> MSDNRRRRREEDDSDSENELPPSSPQQHFRGGMNPVSSPIGSPDMINPEGDDNEVDDVPDIDEVEEQMNEVDLMDDNMYEDYAADHNRDRYDPDQVDDREQQELSLSERRRIDAQLNERDRLLRNVAYIDDEDEEQEGAAQLDEMGLPVQRRRRRRQYEDLENSDDDLLSDMDIDPLREELTLESLSNVKANSYSEWITQPNVSRTIARELKSFLLEYTDETGRSVYGARIRTLGEMNSESLEVNYRHLAESKAILALFLAKCPEEMLKIFDLVAMEATELHYPDYARIHSEIHVRISDFPTIYSLRELRESNLSSLVRVTGVVTRRTGVFPQLKYVKFNCLKCGSILGPFFQDSNEEIRISFCTNCKSKGPFRVNGEKTVYRNYQRVTLQEAPGTVPPGRLPRHREVILLADLVDVSKPGEEVEVTGIYKNNYDGNLNAKNGFPVFATIIEANSIKRREGNTANEGEEGLDVFSWTEEEEREFRKISRDRGIIDKIISSMAPSIYGHRDIKTAVACSLFGGVPKNVNGKHSIRGDINVLLLGDPGTAKSQILKYVEKTAHRAVFATGQGASAVGLTASVRKDPITKEWTLEGGALVLADKGVCLIDEFDKMNDQDRTSIHEAMEQQSISISKAGIVTTLQARCSIIAAANPNGGRYNSTLPLAQNVSLTEPILSRFDILCVVRDLVDEEADERLATFVVDSHVRSHPENDEDREGEELKNNGESAIEQGEDEINEQLNARQRRLQRQRKKEEEISPIPQELLMKYIHYARTKIYPKLHQMDMDKVSRVYADLRRESISTGSFPITVRHLESILRIAESFAKMRLSEFVSSYDLDRAIKVVVDSFVDAQKVSVRRQLRRSFAIYTLGH;> MEGSTGFDGDATTFFAPDAVFGDRVRRFQEFLDTFTSYRDSVRSIQVYNSNNAANYNDDQDDADERDLLGDDDGDDLEKEKKAASSTSLNILPHRIIISLDDLREFDRSFWSGILVEPAYFIPPAEKALTDLADSMDDVPHPNASAVSSRHPWKLSFKGSFGAHALSPRTLTAQHLNKLVSVEGIVTKTSLVRPKLIRSVHYAAKTGRFHYRDYTDATTTLTTRIPTPAIYPTEDTEGNKLTTEYGYSTFIDHQRITVQEMPEMAPAGQLPRSIDVILDDDLVDKTKPGDRVNVVGVFKSLGAGGMNQSNSNTLIGFKTLILGNTVYPLHARSTGVAARQMLTDFDIRNINKLSKKKDIFDILSQSLAPSIYGHDHIKKAILLMLMGGVEKNLENGSHLRGDINILMVGDPSTAKSQLLRFVLNTASLAIATTGRGSSGVGLTAAVTTDRETGERRLEAGAMVLADRGVVCIDEFDKMTDVDRVAIHEVMEQQTVTIAKAGIHTTLNARCSVIAAANPVFGQYDVNRDPHQNIALPDSLLSRFDLLFVVTDDINEIRDRSISEHVLRTHRYLPPGYLEGEPVRERLNLSLAVGEDADINPEEHSNSGAGVENEGEDDEDHVFEKFNPLLQAGAKLAKNKGNYNGTEIPKLVTIPFLRKYVQYAKERVIPQLTQEAINVIVKNYTDLRNDDNTKKSPITARTLETLIRLATAHAKVRLSKTVNKVDAKVAANLLRFALLGEDIGNDIDEEESEYEEALSKRSPQKSPKKRQRVRQPASNSGSPIKSTPRRSTASSVNATPSSARRILRFQDDEQNAGEDDNDIMSPLPADEEAELQRRLQLGLRVSPRRREHLHAPEEGSSGPLTEVGTPRLPNVSSAGQDDEQQQSVISFDNVEPGTISTGRLSLISGIIARLMQTEIFEEESYPVASLFERINEELPEEEKFSAQEYLAGLKIMSDRNNLMVADDKVWRV;> MSQQSSSPTKEDNNSSSPVVPNPDSVPPQLSSPALFYSSSSSQGDIYGRNNSQNLSQGEGNIRAAIGSSPLNFPSSSQRQNSDVFQSQGRQGRIRSSASASGRSRYHSDLRSDRALPTSSSSLGRNGQNRVHMRRNDIHTSDLSSPRRIVDFDTRSGVNTLDTSSSSAPPSEASEPLRIIWGTNVSIQECTTNFRNFLMSFKYKFRKILDEREEFINNTTDEELYYIKQLNEMRELGTSNLNLDARNLLAYKQTEDLYHQLLNYPQEVISIMDQTIKDCMVSLIVDNNLDYDLDEIETKFYKVRPYNVGSCKGMRELNPNDIDKLINLKGLVLRSTPVIPDMKVAFFKCNVCDHTMAVEIDRGVIQEPARCERIDCNEPNSMSLIHNRCSFADKQVIKLQETPDFVPDGQTPHSISLCVYDELVDSCRAGDRIEVTGTFRSIPIRANSRQRVLKSLYKTYVDVVHVKKVSDKRLDVDTSTIEQELMQNKVDHNEVEEVRQITDQDLAKIREVAAREDLYSLLARSIAPSIYELEDVKKGILLQLFGGTNKTFTKGGRYRGDINILLCGDPSTSKSQILQYVHKITPRGVYTSGKGSSAVGLTAYITRDVDTKQLVLESGALVLSDGGVCCIDEFDKMSDSTRSVLHEVMEQQTISIAKAG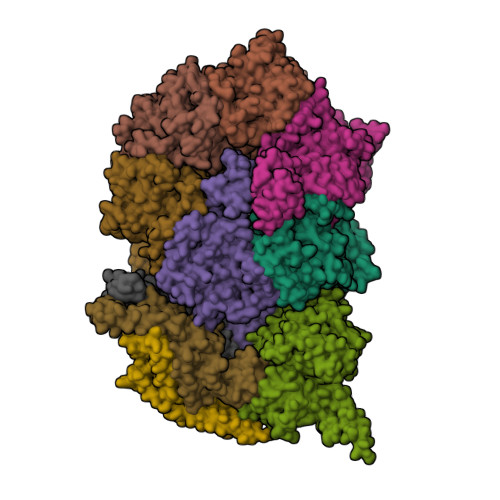IITTLNARSSILASANPIGSRYNPNLPVTENIDLPPPLLSRFDLVYLVLDKVDEKNDRELAKHLTNLYLEDKPEHISQDDVLPVEFLTMYISYAKEHIHPIITEAAKTELVRAYVGMRKMGDDSRSDEKRITATTRQLESMIRLAEAHAKMKLKNVVELEDVQEAVRLIRSAIKDYATDPKTGKIDMNLVQTGKSVIQRKLQEDLSREIMNVLKDQASDSMSFNELIKQINEHSQDRVESSDIQEALSRLQQEDKVIVLGEGVRRSVRLNNRV;> MSFDRPEIYSAPVLQGESPNDDDNTEIIKSFKNFILEFRLDSQFIYRDQLRNNILVKNYSLTVNMEHLIGYNEDIYKKLSDEPSDIIPLFETAITQVAKRISILSRAQSANNNDKDPENTSMDTDSLLLNSLPTFQLILNSNANQIPLRDLDSEHVSKIVRLSGIIISTSVLSSRATYLSIMCRNCRHTTSITINNFNSITGNTVSLPRSCLSTIESESSMANESNIGDESTKKNCGPDPYIIIHESSKFIDQQFLKLQEIPELVPVGEMPRNLTMTCDRYLTNKVIPGTRVTIVGIYSIYNSKNGAGSGRSGGGNGGSGVAIRTPYIKILGIQSDVETSSIWNSVTMFTEEEEEEFLQLSRNPKLYEILTNSIAPSIFGNEDIKKAIVCLLMGGSKKILPDGMRLRGDINVLLLGDPGTAKSQLLKFVEKVSPIAVYTSGKGSSAAGLTASVQRDPMTREFYLEGGAMVLADGGVVCIDEFDKMRDEDRVAIHEAMEQQTISIAKAGITTVLNSRTSVLAAANPIYGRYDDLKSPGDNIDFQTTILSRFDMIFIVKDDHNEERDISIANHVINIHTGNANAMQNQQEENGSEISIEKMKRYITYCRLKCAPRLSPQAAEKLSSNFVTIRKQLLINELESTERSSIPITIRQLEAIIRITESLAKLELSPIAQERHVDEAIRLFQASTMDAASQDPIGGLNQASGTSLSEIRRFEQELKRRLPIGWSTSYQTLRREFVDTHRFSQLALDKALYALEKHETIQLRHQGQNIYRSGV;> MSSPFPADTPSSNRPSNSSPPPSSIGAGFGSSSGLDSQIGSRLHFPSSSQPHVSNSQTGPFVNDSTQFSSQRLQTDGSATNDMEGNEPARSFKSRALNHVKKVDDVTGEKVREAFEQFLEDFSVQSTDTGEVEKVYRAQIEFMKIYDLNTIYIDYQHLSMRENGALAMAISEQYYRFLPFLQKGLRRVVRKYAPELLNTSDSLKRSEGDEGQADEDEQQDDDMNGSSLPRDSGSSAAPGNGTSAMATRSITTSTSPEQTERVFQISFFNLPTVHRIRDIRSEKIGSLLSISGTVTRTSEVRPELYKASFTCDMCRAIVDNVEQSFKYTEPTFCPNPSCENRAFWTLNVTRSRFLDWQKVRIQENANEIPTGSMPRTLDVILRGDSVERAKPGDRCKFTGVEIVVPDVTQLGLPGVKPSSTLDTRGISKTTEGLNSGVTGLRSLGVRDLTYKISFLACHVISIGSNIGASSPDANSNNRETELQMAANLQANNVYQDNERDQEVFLNSLSSDEINELKEMVKDEHIYDKLVRSIAPAVFGHEAVKKGILLQMLGGVHKSTVEGIKLRGDINICVVGDPSTSKSQFLKYVVGFAPRSVYTSGKASSAAGLTAAVVRDEEGGDYTIEAGALMLADNGICCIDEFDKMDISDQVAIHEAMEQQTISIAKAGIHATLNARTSILAAANPVGGRYNRKLSLRGNLNMTAPIMSRFDLFFVILDDCNEKIDTELASHIVDLHMKRDEAIEPPFSAEQLRRYIKYARTFKPILTKEARSYLVEKYKELRKDDAQGFSRSSYRITVRQLESMIRLSEAIARANCVDEITPSFIAEAYDLLRQSIIRVDVDDVEMDEEFDNIESQSHAASGNNDDNDDGTGSGVITSEPPADIEEGQSEATARPGTSEKKKTTVTYDKYVSMMNMIVRKIAEVDREGAEELTAVDIVDWYLLQKENDLGSLAEYWEERRLAFKVIKRLVKDRILMEIHGTRHNLRDLENEENENNKTVYVIHPNCEVLDQLEPQDSS;> MSAALPSIQLPVDYNNLFNEITDFLVTFKQDTLSSDATRNENEDENLDAENIEQHLLEKGPKYMAMLQKVANRELNSVIIDLDDILQYQNEKFLQGTQADDLVSAIQQNANHFTELFCRAIDNNMPLPTKEIDYKDDVLDVILNQRRLRNERMLSDRTNEIRSENLMDTTMDPPSSMNDALREVVEDETELFPPNLTRRYFLYFKPLSQNCARRYRKKAISSKPLSVRQIKGDFLGQLITVRGIITRVSDVKPAVEVIAYTCDQCGYEVFQEVNSRTFTPLSECTSEECSQNQTKGQLFMSTRASKFSAFQECKIQELSQQVPVGHIPRSLNIHVNGTLVRSLSPGDIVDVTGIFLPAPYTGFKALKAGLLTETYLEAQFVRQHKKKFASFSLTSDVEERVMELITSGDVYNRLAKSIAPEIYGNLDVKKALLLLLVGGVDKRVGDGMKIRGDINVCLMGDPGVAKSQLLKAICKISPRGVYTTGKGSSGVGLTAAVMKDPVTDEMILEGGALVLADNGICCIDEFDKMDESDRTAIHEVMEQQTISISKAGINTTLNARTSILAAANPLYGRYNPRLSPLDNINLPAALLSRFDILFLMLDIPSRDDDEKLAEHVTYVHMHNKQPDLDFTPVEPSKMREYIAYAKTKRPVMSEAVNDYVVQAYIRLRQDSKREMDSKFSFGQATPRTLLGIIRLSQALAKLRLADMVDIDDVEEALRLVRVSKESLYQETNKSKEDESPTTKIFTIIKKMLQETGKNTLSYENIVKTVRLRGFTMLQLSNCIQEYSYLNVWHLINEGNTLKFVDDGTMDTDQEDSLVSTPKLAPQTTASANVSAQDSDIDLQDA;> MYGDLGNKLVLEAKRTKQLYARSNQDVNLPMYHEDIIRNILKEVSNLRKNTEYLKEQQQLGMLDDKVAKCQYFVTLLCMERNKRCLLAYQRLRTDILDSMAWNNNGLDLMSSITFSQQDTNNLSHQEQEYLKEYCDLITDLKSGDLVDIDLSGSLVPPSDAFIDVRVLKDAGEIQTEYGVFNLIKDSQFFVQQSDVERLIQQGYLQLI;> MSLPAHLQQTFSPEEIQFIVENEPIKIFPRITTRQKIRGDDRGTGNHTRWQLITTDDKALNNMVAMRSTEVVLWIALLLKQQSKCSIVAPQWLTTKELDRKIQYEKTHPDRFSELPWNWLVLARILFNKAKDDFHDPIHELRGKIQDLREIRQIKVLKGLKYLNESHLQLDNLSLLEINELRPFITEIMDKLREIHTASLTAGTENDEEEFNI;> MGYYDIDDVLADGTEFPCKFQYDIPGLGYLENNPGRPITKNTKLSLPLWLARILAIVGGDEALVDEEPVPFVELLPPDMFSTKVMNAIKTDPVALDLHSINSHFFSLAIKWIMLFSEKELANVVSELLLQRAQELNHHASSLSIDLNADSTGKNSANTNIATSTFLLKLEEMEKEIYKKSHESYKDTKRWMFKK;> MDINIDDILAELDKETTAVDSTKITQGSSSTTHRDANTIVGSSLDLNDKTQIYVSPQQDFSDLMKSWKNERCSPELLPYPHQLMKRLLNRISMQSQLIENISMGFLDMQNASNANPPMPNESKLPLLCMETELERLKFVIRSYIRCRLSKIDKFSLYLRQLNEDENSLISLTDLLSKDEIKYHDTHSLIWLKLVNDSILKYMPEELQAINDTEGSVNMIDEPDWNKFVFIHVNGPPDGKWNEDPLLQENEFGKPCYTVTIPDLKEEVELTIGSIYVMRYEVIRDLLRDDKVALI;> MYYGISQFSEAYNKILRNSSSASSCQLVIFVSCLNIDALCATKMLSLLFKKQLVQSQIVPIFGYSELRRHYSQLDDNINSLLLVGFGGVIDLEAFLEIDPQEYVIDTDEKSGEQSFRRDIYVLDAHRPWNLDNIFGSQIIQCFDDGTVDDTLGEEKEAYYKLLELDEESGDDELSGDENDNNGGDDEATDADEVTDEDEEDEDETISNKRGNSSIGPNDLSKRKQRKKQIHEYEGVLEEYYSQGTTVVNSISAQIYSLLSAIGETNLSNLWLNILGTTSLDIAYAQVYNRLYPLLQDEVKRLTPSSRNSVKTPDTLTLNIQPDYYLFLLRHSSLYDSFYYSNYVNAKLSLWNENGKKRLHKMFARMGIPLSTAQETWLYMDHSIKRELGIIFDKNLDRYGLQDIIRDGFVRTLGYRGSISASEFVEALTALLEVGNSTDKDSVKINNDNNDDTDGEEEEDNSAQKLTNLRKRWVSNFWLSWDALDDRKVELLNRGIQLAQDLQRAIFNTGVAILEKKLIKHLRIYRLCVLQDGPDLDLYRNPLTLLRLGNTLIECCAESEDKQLLPMVLASIDENTDTYLVAGLTPRYPRGLDTIHTKKPILNNFSMAFQQITAETDAKVRIDNFESSIIEIRREDLSPFLEKLTLSGLL> GPSGSELADLAEETLKIFRANKFELGLVPDIP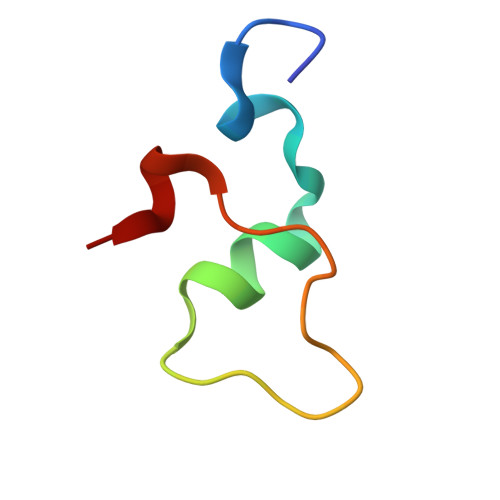PPPALVA> MFGGIENVKAAEPKVYQFDFGSGSMEPGYIGVRASDRYDRSKGYGFQTPENMRD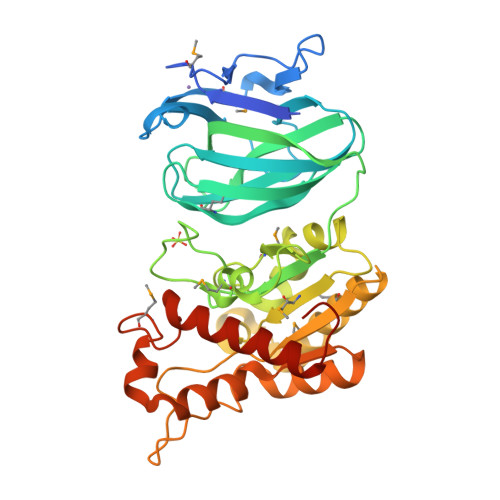VAASGAGVKSDAVEFLAYGTKSNNTFNVDLPNGLYEVKVTLGNTARASVAAEGVFQVINMTGDGAEDTFQIPVTDGQLNLLVTEGKAGTAFTLSALKIKKLSDQPVTNRTIYVGGDSTVCNYYPLNSSKQAGWGQMLPHYIDKHTFQVRNMASGGQIARGFRNDGQLEAILKYIKPGDYFMLQLGINDTNPKHKESEAEFKEVMRDMIRQVKAKGADVILSTPQGRATDFTSEGIHSSVNRWYRASILALAEEEKTYLIDLNVLSSAYFTSIGPERTLGLYMDGDTLHPNRAGADALARLAVQELKRQGIAGFLEHHHHHH> MTAGYEPCWLRYERKDQYSRLRFEEIVAKRTSPIFQAVVEELQKGLRSMMEIEPQVVQEVNETANSIWLGTLEDEEFERPLEGTLVHPEGYVIRSDVDDGPFRIYIIGKTDAGVLYGVFHFLRLLQMGENIAQLSIIEQPKNRLRMINHWDNMDGSIERGYAGRSIFFVDDQFVKQNQRIKDYARLLASVGINAISINNVNVHKTETKLITDHFLPDVAEVADIFRTYGIKTFLSINYASPIEIGGLPTADPLDPEVRRWWKETAKRIYQYIPDFGGFVVKADSNFRPGPFTYGRDHAEGANMLAEALAPFGGLVIWRCFVYNCQQDWRDRTTDRAKAAYDHFKPLDGQFRENVILQIKNGPMDFQVREPVSPLFGAMPKTNQMMEVQITQEYTGQQKHLCFLIPQWKEVLDFDTYAKGKGSEVKKVIDGSLFDYRYSGIAGVSNIGSDPNWTGHTLAQANLYGFGRLAWNPDLSAEEIANEWVVQTFGDDSQVVETISWMLLSSWRIYENYTSPLGVGWMVNPGHHYGPNVDGYEYSHWGTYHYADRDGIGVDRTVATGTGYTAQYFPENAAMYES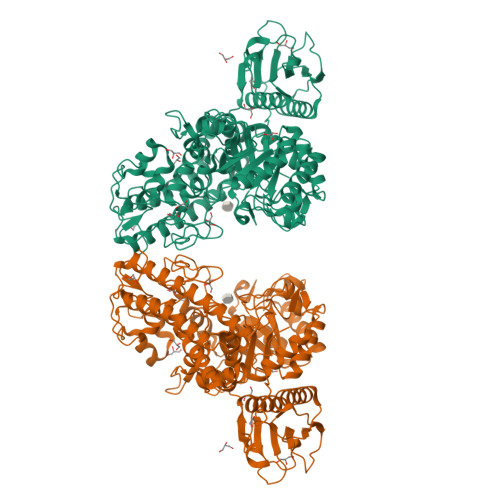LDTCPDELLLFFHHVPYTHRLHSGETVIQHIYNTHFEGVEQAKQLRKRWEQLKGKIDEKRYHDVLERLTIQVEHAKEWRDVINTYFYRKSGIDDQYGRKIYR> SNAMKEMKAIQFDQFGPPKVLKLVDTPTPEYRKNQMLIKVHAASLNPIDYKTRNGSGFVAKKLKNNLPSGLGYDFSGEVIELGSDVNNVNIGDKVMGIAGFPDHPCCYAEYVCASPDTIIQKLEKLSFLQAASLPTAGLTALQALNQAEVKQGDVVLIHAGAGGVGHLAIQLAKQKGTTVITTASKRNHAFLKALGAEQCINYHEEDFLLAISTPVDAVIDLVGGDVGIQSIDCLKETGCIVSVPTITAGRVIEVAKQKHRRA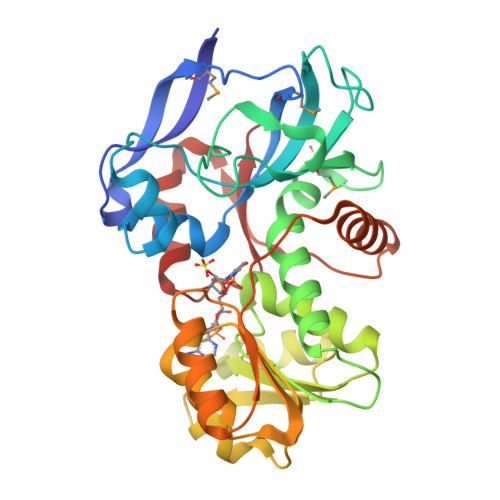FGLLKQFNIEELHYLGKLVSEDKLRIEISRIFQLSEAVTAHELLETGHVRGKLVFKVR>[4x]MGACPPKAKGPWAQLQKLLISWPVGEQDWEQYRDRVNMLQQERIRDSPLLQAAKENDLRLLKILLLNQSCDFQQRGAVGETALHVAALYDNLEAATLLMEAAPELAKEPALCEPFVGQTALHIAVMNQNLNLVRALLARGASVSARATGAAFRRSPHNLIYYGEHPLSFAACVGSEEIVRLLIEHGADIRAQDSLGNTVLHILILQPNKTFACQMYNLLLSYDEHSDHLQSLELVPNHQGLTPFKLAGVEGNTVMFQHLMQKRKHVQWTCGPLTSTLYDLTEIDSWGEELSFLELVVSSKKREARQILEQTPVKELVSFKWKKYGRPYFCVLASLYILYMICFTTCCIYRPLKLRDDNRTDPRDITILQQKLLQEAYVTHQDNIRLV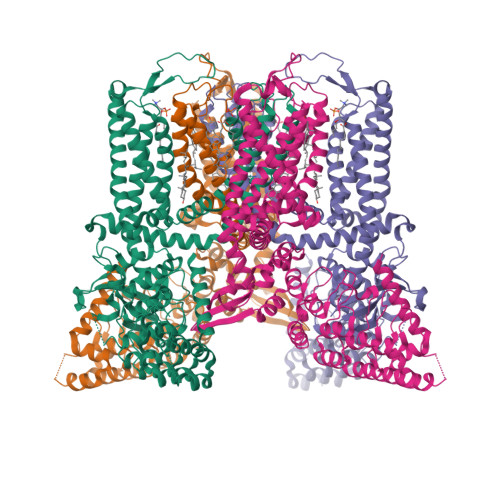GELVTVTGAVIILLLEIPDIFRVGASRYFGQTILGGPFHVIIITYASLVLLTMVMRLTNMNGEVVPLSFALVLGWCSVMYFARGFQMLGPFTIMIQKMIFGDLMRFCWLMAVVILGFASAFHITFQTEDPNNLGEFSDYPTALFSTFELFLTIIDGPANYSVDLPFMYCITYAAFAIIATLLMLNLFIAMMGDTHWRVAQERDELWRAQVVATTVMLERKMPRFLWPRSGICGYEYGLGDRWFLRVENHHDQNPLRVLRYVEAFKCSDKEDGQEQLSEKRPSTVESGMLSRASVAFQTPSLSRTTSQSSNSHRGWEILRRNTLGHLNLGLDLGEGDGEEVYHFTETSQVAPA>MSLVKKSSNVIAAVVSSVRTNFAQQILDGIQEEAHKNGYNLIIVYSGSADPEEQKHALLTAIERPVMGILLLSIALTDDNLQLLQSSDVPYCFLSMGFDDDRPFISSDDEDIGYQATNLLINEGHRQIGIAGIDQYPYTGRKRLAGYKKALKEANIAINQEWIKPGDYSYTSGEQAMKAFGKNTDLTGIIAASDMTAIGILNQASSFGIEVPKDLSIVSIDGTEMCKITRPQLTSISQDFF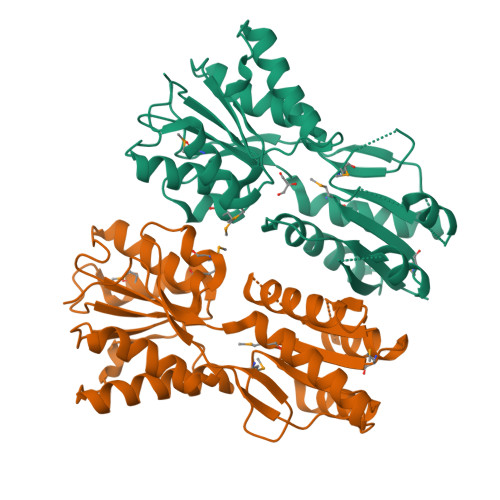QMGVTGVQQIHQSVKNGSNRIVSQQFIPVNPVIRKSTARLGEGHHHHHH[2x]>[2x]GSHMAVQIGFLLFPEVQQLDLTGPHDVLASLPDVQVHLIWKEPGPVVASSGLVLQATTSFADCPPLDVICIPGGTGVGALMEDPQALAFIRQQAARARYVTSVCTGSLVLGAAGLLQGKRATTHWAYHELLAPLGAIPVHERVVRDGNLLTGAGITAGIDFALTLAAELFDAATAQRVQLQLEYAPAPPFNAGSPDTAPASVVQQARQRAADSLHKRREITLRAAARLAAG

Here, we address each of these questions in a study of diffuse scattering from crystalline isocyanide hydratase (ICH). We selected the ICH system because it diffracts x-rays to atomic resolution at ambient temperature, has clearly visible diffuse features in ambient temperature x-ray diffraction datasets, and displays large concerted motion of an α-helix that is modulated by the chemical state of the active site nucleophile. Upon formation of the catalytic thioimidate intermediate, this helix becomes more mobile and permits water to enter the active site and complete the reaction.

Engineered mutations at residue 150 (e.g., G150A, G150T) also favor shifted conformations of the helix to varying degrees. The refined WT and G150A ICH models are also highly similar (∼0.05–0.07 Å Cα RMSD). In addition, the six WT and G150A datasets show ∼2σ difference (mFo − DFc) electron density features around the mobile helix that indicate a minor population (<10% occupancy) of the shifted helix conformation. The near-identical WT and G150A ICH dimeric protein structures (Cα RMSD ∼ 0.06 Å) provide an opportunity to evaluate the cross correlation coefficient (CCCross) of their diffuse scattering maps. The CCCross for WT-1, for example, can be calculated as the average CC of CC(WT-1, G150A-1), CC(WT-1, G150A-2), and CC(WT-1, G150A-3). We find that the CCCross is ≥0.83 for every WT and G150A dataset, and each data pair within the set of replicate WT and G150A datasets also has CC ≥ 0.8, as shown in orange-colored cells in Table S5. The high cross correlation between WT and G150A diffuse datasets provides additional evidence that protein-derived diffuse scattering is the dominant feature in the processed diffuse anisotropic maps and is consistent with the minor differences in the crystal structures refined against the Bragg data. In general, the CCLLM values are higher and σ values are lower for the Refmac5 anisotropic ADP models compared to those refined in PHENIX.> SVFAYESSVHSTNVLLSLNDQRKKDVLCDVTIFVEGQRFRAHRSVLAACSSYFHSRIVGQADGELNITLPEEVTVKGFEPLIQFAYTA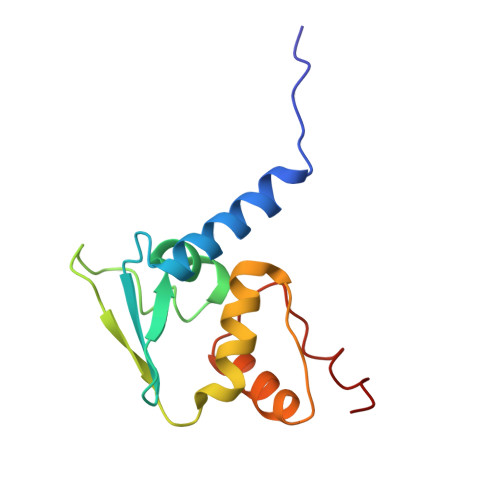KLILSKENVDEVCKCVEFLSVHNIEESCFQFLKF>GSHMAAGGDHGSPDSYRSPLASRYASPEMCFVFSDRYKFRTWRQLWLWLAEAEQTLGLPITDEQIQEMKSNLENIDFKMAAEEEKRLRHDVMAHVHTFGHCCPKAAGIIHLGATSCYVGDNTDLIILRNALDLLLPKLARVISRLADFAKERASLPTLGFTHFQPAQLTTVGKRCCLWIQDLCMDLQNLKRVRDDLRFRGVKGTTGTQASFLQLFEGDDHKVEQLDKMVTEKAGFKRAFIITGQTYTRKVDIEVLSVLASLGASVHKICTDIRLLANLKEMEEPFEKQQIGSSAMPYKRNPMRSERCCSLARHLMTLVMDPLQTASVQWFERTLDDSANRRICLAEAFLTADTILNTLQNISEGLVVYPKVIERRIRQELPFMATENIIMAMVKAGGSRQDCHEKIRVLSQQAASVVKQEGGDNDLIERIQADAYFSPIHSQLDHLLDPSSFTGRASQQVQRFLEEEVYPLLKPYESVMKVKAELCL[8x]

ADSL is involved in the de novo purine biosynthesis and recycling pathways in which it catalyses the conversion of 5-aminoimidazole-(N-succinylocarboxamide) (SAICAR) to 5-aminoimidazole-4-carboxamide ribotide (AICAR) and the conversion of succinyladenosine monophosphate (SAMP) to adenosine monophosphate (AMP), respectively. Both reactions are β-eliminations in which fumarate is released. Domain 1 (residues 22–112) and domain 2 form the base and one side of the active site thus creating a binding cleft for the substrate, while domain 3 (residues 365–450) resembles a lid which sits on top of the active site.

Co-crystallisation of nADSL with its other products AICAR and fumarate (AICAR/fumarate) yielded a different crystal form than seen for the apo and AMP/fumarate bound crystals. In this new crystal form, two nADSL tetramers are present in the asymmetric unit (tetramer ABCD and tetramer EFGH) in contrast to the single tetramer present in the apo and AMP/fumarate bound structures. More specifically, domain 3 is tilted by around 20–25° towards the active site in two protomers of tetramer EFGH (chains G and F) and in one protomer of tetramer ABCD (chain D). As such, the conformation of domain 3 in the G chain will be referred to as the ‘closed conformation’ in the remainder of the text while the conformation in chain F will be referred to as the ‘semi-closed conformation’. However, since domain 3 closure occurs through a rigid body movement involving two hinge points near its N- and C-terminus (Leu377 and Phe449), the central region of the domain (including residue 429) is structurally identical in all three conformations. However, in the AICAR/fumarate bound nADSL structure, Arg396 is inserted into the active site and forms part of a hydrogen bond network involving residues from domain 1 in the semi-closed conformation and the catalytic C3-loop (belonging to domain 2) in the fully closed conformation. Indeed, electron density for the C3-loop is only clearly defined in the protomers of the AICAR/fumarate bound nADSL structure where domain 3 adopts the closed or semi-closed conformation. In those active sites in which the domain adopts the semi-closed or open conformation, the reverse enzymatic reaction appeared to have occurred in the crystals since they all have substrate SAICAR bound. In contrast, the adjacent Ser290 residue directly H-bonds with the carboxyl group of fumarate thus being more favourable situated to act as catalytic base.>MPLKNRLLARLSCVAAVVAATAAVAPLTLVSTAHAAAPQVRTSAPGYYRMLLGDFEITALSDGTVALPVDKRLNQPAPKTQSALAKSFQKAPLETSVTGYLVNTGSKLVLVDTGAAGLFGPTLGRLAANLKAAGYQPEQVDEIYITHMHPDHVGGLMVGEQLAFPNAVVRADQKEADFWLSQTNLDKAPDDESKGFFKGAMAS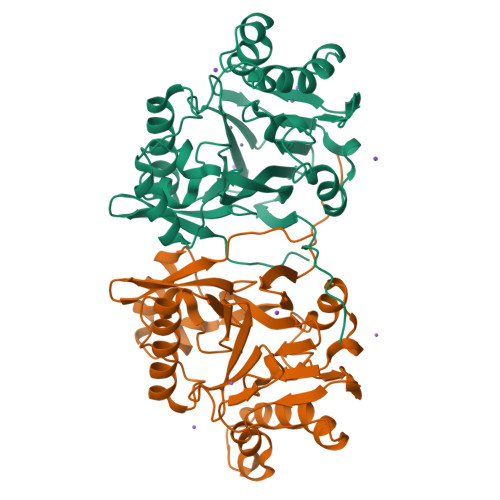LNPYVKAGKFKPFSGNTDLVPGIKALASHGHTPGHTTYVVESQGQKLALLGDLILVAAVQFDDPSVTTQLDSDSKSVAVERKKAFADAAKGGYLIAASHLSFPGIGHIRAEGKGYRFVPVNYSVVNPK[2x]>PPSVFAEVPQAQPVLVFKLTADFREDPDPRKVNLGVGAYRTDDCHPWVLPVVKKVEQKIANDNSLNHEYLPILGLAEFRSCASRLALGDDSPALKEKRVGGVQSLGGTGALRIGADFLARWYNGTNNKNTPVYVSSPTWENHNAVFSAAGFKDIRSYRYWDAEKRGLDLQGFLNDLENAPEFSIVVLHACAHNPTGIDPTPEQWKQIASVMKHRFLFPFFDSAYQGFASGNLERDAWAIRYFVSEGFEFFCAQSFSKNFGLYNERVGNLTVVGKEPESILQVLSQMEKIVRITW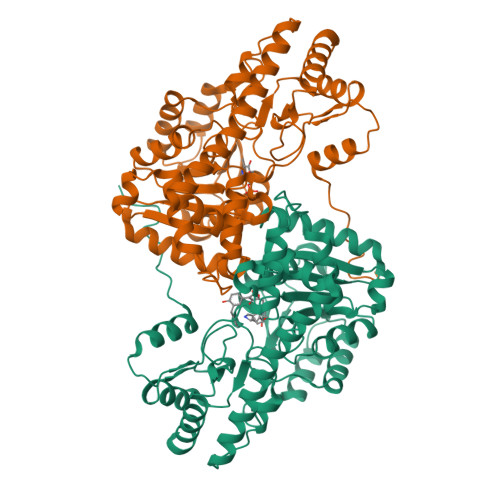SNPPAQGARIVASTLSNPELFEEWTGNVKTMADRILTMRSELRARLEALKTPGTWNHITDQIGMFSFTGLNPKQVEYLVNEKHIYLLPSGRINVSGLTTKNLDYVATSIHEAVTKIQ[2x]> GSSHEAAAAQQHNSGTQHTVSGSQQEGQQRKQHHSSKPTASMPRPHSDWQIPDRYEIRHLIGTGSYGHVCEAYDKLEKRVVAIKKILRVFEDLIDCKRILREIAILNRLNHDHVVKVLDIVIPKDVEKFDELYVVLEIADSDF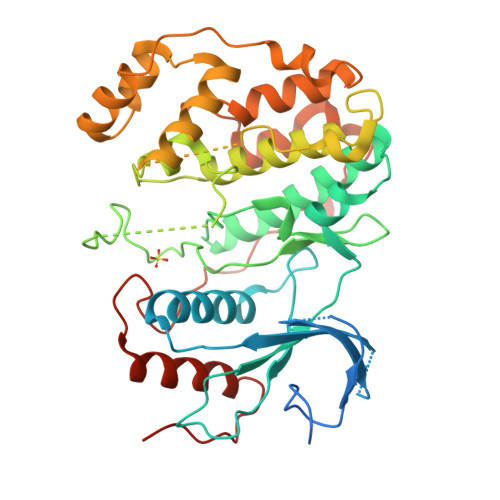KKLFRTPVYLTELHIKTLLYNLLVGVKYVHSAGILHRDLKPANCLVNQDCSVKVCDFGLARTVDYPENGNSQLPISPREDDMNLVTFPHTKNLKRQLTGHVVTRWYRAPELILLQENYTEAIDVWSIGCIFAELLNMIKENVAYHADRGPLFPGSSCFPLSPDQKAGNDFKFHTRGNRDQLNVIFNILGTPSEEDIEALEKEDAKRYIRIFPKREGTDLAERFPASSADAIHLLKRMLVFNPNKRITINECLAHPFFKEVRIAEVETNATEKVRLPFNDWMNMDEPQLRYAFVKEIQRYHPEIQLPRRSPNRASS> GSFIDIEFPEWFHEGLSRHQAENLLMGKDIGFFIIRASQSSPGDFSISVRHEDDVQHFKVMRDTKGNYFLWTEKFPSLN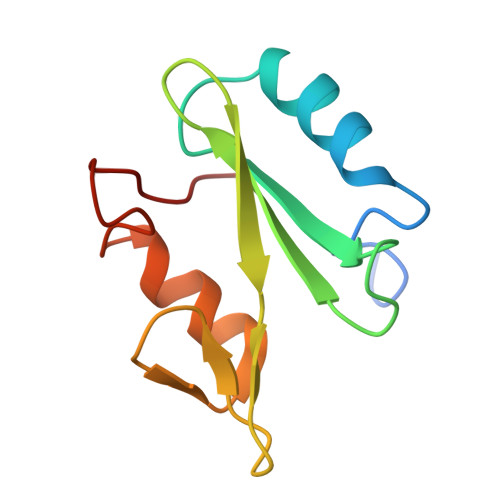KLVDYYRTTSISKQKQVFLRD PSTPIP1 is an adaptor protein expressed in most immune cell lineages. It presents two structural domains in its sequence, an N-terminal Fer/CIP4 homology-Bin/Amphiphysin/Rvs (F-BAR) domain and a C-terminal SH3 domain, connected by a linker region. The F-BAR domain of PSTPIP1 binds to the PEST subfamily of protein tyrosine phosphatases (PTPs): PTPN12, also known as PTP-PEST, PTPN18, and the lymphoid phosphatase (LYP), encoded by the gene PTPN22. Positively charged residues on the concave surface of F-BAR domains interact with the polar heads of the phospholipids in the cellular membrane.

We determined the previously unknown structure of the isolated F-BAR domain of PSTPIP1. To better understand the molecular basis of the physiological function of PSTPIP1 in the immune system, and its role in autoinflammatory diseases, we elucidated the 3D structure of the F-BAR domain (residues 1–289) using X-ray crystallography. Initially, we solved the structure of the G258A mutant, and subsequently that of the wild type protein. The two structures were almost identical. After superimposition, the root mean square deviation (rmsd) between all the equivalent Cα atoms was 0.275 Ǻ, which was similar to the estimated errors of the coordinates of the structures (0.23–0.24 Ǻ). The asymmetric unit of the crystal contains two molecules of PSTPIP1 that form the characteristic elongated crescent-shape of F-BAR dimers. The concave side of the F-BAR dimer is overall electropositive and contains two clusters of basic residues in each protomer, one in the core region, and the other near the tip of the wing. On the other hand, the central area of the convex surface has strong electronegative character due to the presence of multiple acidic residues. Large acidic surfaces are observed in the F-BAR domains of other proteins, such as Cdc15, growth arrest-specific 7 (GAS7), and formin-binding protein 17 (FBP17), but are absent in several F-BAR domains. The residues of PSTPIP1 critical for binding to PEST phosphatases (see above) are located in this electronegative area, supporting the notion that the acidic convex area is important for PSTPIP1 function. Finally, the conformation of the PSTPIP1 residues involved in LYP binding is very similar in the free and bound structures.

>[2x]GSHMMPQLQFKDAFWCRDFTAHTGYEVLLQRLLDGRKMCKDMEELLRQRAQAEERYGKELVQIARKAGGQTEINSLRASFDSLKQQMENVGSSHIQLALTLREELRSLEEFRERQKEQRKKYEAVMDRVQKSKLSLYKKAMESKKTYEQKCRDADDAEQAFERISANGHQKQVEKSQNKARQCKDSATEAERVYRQSIAQLEKVRAEWEQEHRTTCEAFQLQEFDRLTILRNALWVHSNQLSMQCVKDDELYEEVRLTLEGCSIDADIDSFIQAKSTGTEPPAPVPYQNYYD>[4x]MADLNWISSALIKERPSADAVLAKAVLAAREQLGLTQLELAGIVGVDRSAISRWKTQGLRVDSKTGELALLLVRVYRALYALFGGQQEDMRHFLRTPNHHLAGEPLALMGQVQGLVHVLEYLDAIRGKV;>MGSSHHHHHHSQDPSEIWRQCKGERHIRPLQGRLVRLVESQEQVATLQLVDTLEEQALLEELLESSKPPVPADAEPLHYLLKTPFRYPPLRWGSRFGRRHEPSLFYAALKLETAMAESAYYRCVLWSGMVVPPPSGRILSEHASFEAGWKVERGIRLQAPPFSDHEAALTDIADYRAPQELGSAMRSAGVQAFEYRSARCPERGCNVALFTPAAFTEKRPRNLTPWLCETTAGYVAFKPAHVPGSPKIFSWELFLVDGKLPHPA[2x]

Here, we show that the NatR–NatT TA system, which is part of the core genome of the human pathogen Pseudomonas aeruginosa, generates drug-tolerant persisters by specifically depleting nicotinamide dinucleotides. We show that NatT is an NAD phosphorylase, which leads to the depletion of both NAD and NADP in a subpopulation of cells. NatT function is tightly controlled by NatR, which is both an anti-toxin and an auxiliary factor required for toxin stability. NatT belongs to a subgroup of RES domain proteins that have adopted a Flap region mediating its interaction with the anti-toxin NatR.

To elucidate the molecular details of NatT activity and its control by NatR, we solved the crystal structure of the NatR–NatT complex. NatR–NatT adopts a hexameric structure with two central NatT molecules flanked by two dimers of NatR (NatR’ and NatR”). NatT is composed of a peripheral ring of α-helices and two central β-sheets that form a cavity (Fig. EV3B). Although NatT is structurally similar to other RES domain proteins it harbors an additional helix–loop–helix domain (hereafter referred to as ‘Flap’), which provides most of the interaction surface between NatT and NatR’ (C and EV3B–D). The Flap contains several conserved negative charges (E26, D38, E42, and E47), which form electrostatic interactions with positive residues in helices α1, α4, and α7 of NatR’. For example, E29 of NatT forms an electrostatic interaction with R119, the last but two amino acids of the C-terminal helix α7 of NatR’. Moreover, a well-defined tetrahedral atomic density modeled as a phosphate molecule was found in the interface between the Flap and NatR’, in close vicinity of residue E29 (E and EV3B). Residues R82, Y108, Y162, and R186 coordinate a second phosphate molecule in the active site of NatT, positioned next to the nicotinamide group of NAD+, that likely participates directly in the cleavage of NAD+ (Fig. EV3B). In the NatR–NatT complex, the C-terminal helix α7 of NatR’ extends all the way into the substrate-binding cavity of NatT, indicating that NatR’ controls toxin activity by blocking substrate access and that dynamic repositioning of α7 and NatR’ is likely required to activate NatT. Of note, the Flap is tightly sandwiched between NatR’ and the adjacent NatT protomer, restricting Flap movement and keeping the active site pocket occluded by the C-terminus of NatR’.>[4x]AKNIQAIRGMNDYLPGETAIWQRIEGTLKNVLGSYGYSEIRLPIVEQTPLFKRAIGEVTDVVEKEMYTFEDRNGDSLTLRPEGTAGCVRAGIEHGLLYNQEQRLWYIGPMFRHERPQKGRYRQFHQLGCEVFGLQGPDIDAELIMLTARWWRALGISEHVTLELNSIGSLEARANYRDALVAFLEQHKEKLDEDCKRRMYTNPLRVLDSKNPEVQA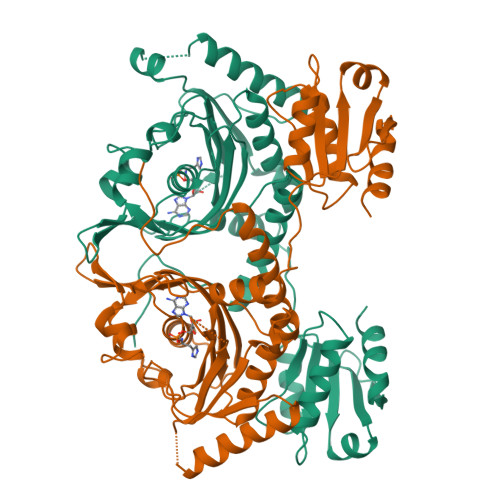LLNDAPALGDYLDEESREHFAGLCKLLESAGIAYTVNQRLVRGLDYYNRTVFEWVTNSLGSQGTVCAGGRYDGLVEQLGGRATPAVGFAMGLERLVLLVQAVNPEFKADPVVDIYLVASGADTQSAAMALAERLRDELPGVKLMTNHGGGNFKKQFARADKWGARVAVVLGESEVANGTAVVKDLRSGEQTAVAQDSVAAHLRTLLG> QPRRPALRQCCNQLRQVDRPCVCPVLRQAAQQVLQRQIIQGPQQLRRLFDAARNLPNI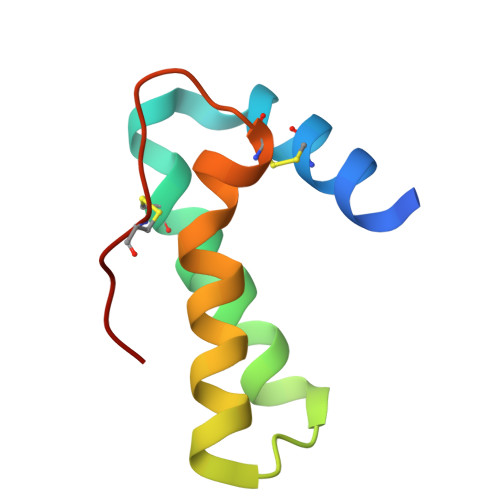CNIPNIGACPFRAW>[2x]MSGTSSEEAKEAIIAMLKEWYDAMNEGDMEKLRSLVDPDASFVDARTNQVYDKDQFLQMIKEALEQDLKVEVKSIDI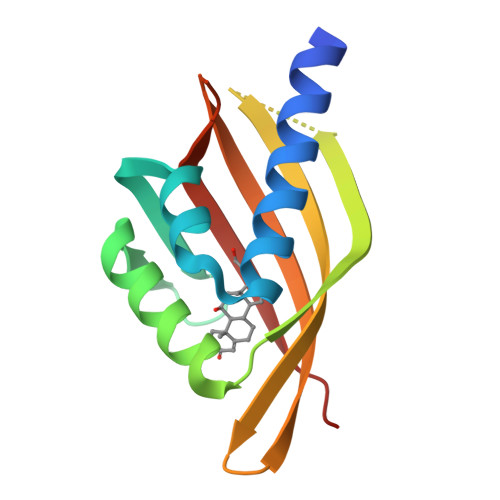EQQPDGDVVIVKVKVRATMVRNGQEHVFEVVDTYEFRRKGDSWKIVKLVSEITQLGSG>SNAMNIEIKDTLISEEQLQEKVKELALQIERDFEGEEIVVIAVLKGSFVFAADLIRHIKNDVTIDFISASSYGNQTETTGKVKLLKDIDVNITGKNVIVVEDIIDSGLTLHFLKDHFFMHKPKALKFCTLLDKPERRKVDLTAEYVGFQIPDEFIVGYGIDCAEKYRNLPFIASVVTEESYNLK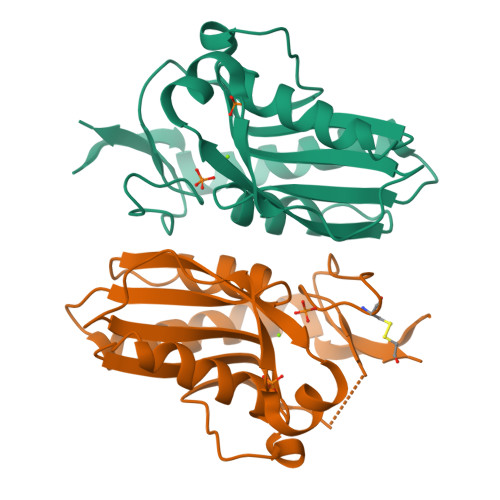SR[5x]> STSAASSSNYCNQMMKSRNLTKDRCKPVN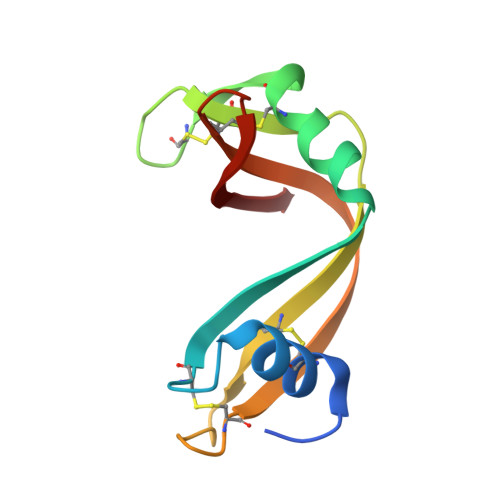TFVHESLADVQAVCSQKNVACKNGQTNCYQSYSTMSITDCRETGSSKYPNCAYKTTQANKHIIVACEGNPYVPVHFDASV> SEADEMAKAL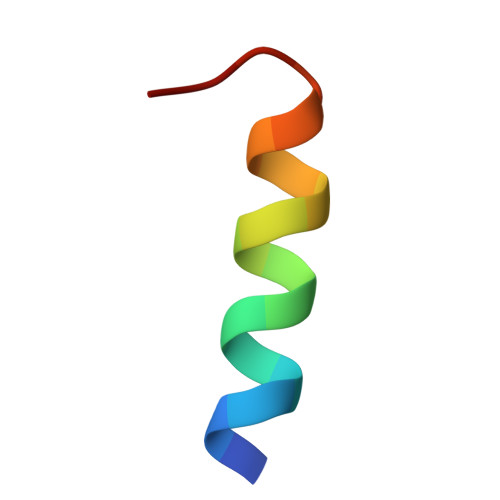EAELNDLM> MARIIVVTSGKGGVGKTTSSAAIATGLAQKGKKTVVIDFAIGLRNLDLIMGCERRVVYDFVNVIQGDATLNQALIKDKRTENLYILPASQTRDKDALTREGVAKVLDDLKAMDFEFIVCDSPAGIETGALMALYFADEAIITTNPEVSSVRDSDRILGILASKSRRAENGEEPIKEHLLLTRYNPGRVSRGDMLSMEDVLEILRIKLVGVIPED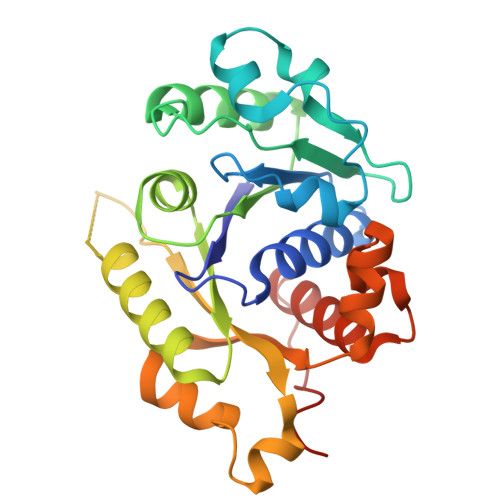QSVLRASNQGEPVILDINADAGKAYADTVERLLGEERPFRFIEEEK(3S)-3-({3-[(1R)-3-amino-1-hydroxypropyl]phenoxy}methyl)hexan-1-ol 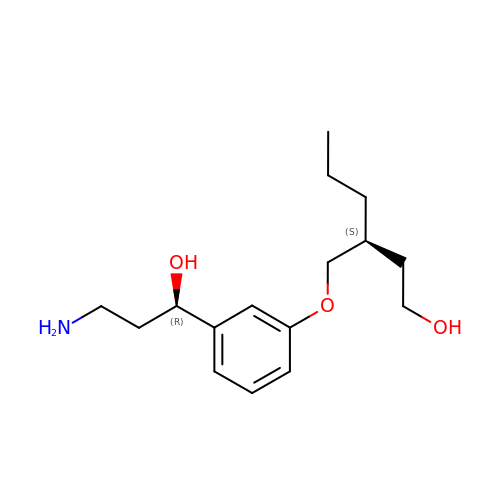| C16 H27 N O3 | UARCALHUUKLSEU-XJKSGUPXSA-N A deazaflavin-dependent nitroreductase (Ddn) from Mycobacterium tuberculosis catalyzes the reduction of nitroimidazoles such as PA-824, resulting in intracellular release of lethal reactive nitrogen species. The N-terminal 30 residues of Ddn are functionally important but are flexible or access multiple conformations, preventing structural characterization of the full-length, enzymatically active enzyme. The split barrel-like fold is characterized by a central six-stranded antiparallel β barrel in a Greek key topology with four α helices: A at the N terminus (the putative helix removed for Ddn structure determination), B after an extended loop between strands β3 and β4, and C and D between strands β5 and β6. The identification of these residues and the lack of classic catalytic residues in the active site suggest that Ddn functions primarily by precisely orienting PA-824 for efficient direct hydride transfer from F420 and potentially through additional transition-state stabilization.

Well-dispersed signals for 113 of 114 nonproline residues were observed by 1H-15N-HSQC NMR spectroscopy for uniformly 15N-labeled NΔ30 Ddn protein, suggesting a well-defined three-dimensional structure. This sample also showed significant chemical shift perturbation upon addition of oxidized or reduced coenzyme F420, demonstrating tight binding of the coenzyme and suggesting that this construct adopts a physiologically relevant form. As expected (Manjunatha et al., 2006a; Taylor et al., 2010), the backbone trace shows high similarity to proteins in the split barrel-like family of flavin-binding proteins. The initial structure was then used to solve the structure of the longer NΔ30 construct by molecular replacement based on a 1.55 Å data set (Apo-1 in Table 1) and of a 1.85 Å resolution NΔ33 crystal (P3221 space group; Apo-2 in Table 1). All but the first five amino-terminal residues could be built into the electron density for both crystal forms (36–151 and 39–151, respectively). The asymmetric units (ASUs) for the Apo-1 and Apo-2 crystals both contain single molecules with similar structures (root-mean-square deviation [rmsd] is 0.96 Å). This alignment omits 14 of 113 shared Cα atoms because of conformational differences in the same regions that differ upon coenzyme binding. In Apo-1 and Apo-2, α helix D is highly disrupted, with repositioning of residues 129–144 relative to the holo-enzyme structures complementing movement of the post-β3 loop. In Apo-1, the side chain of Y136 is flipped away from the F420 binding site, with the oxygen atom moving 19 Å relative to the Holo-1 structure.

> GRNDGEGLGGTFQKIPVALLTTTGRKTGQPRVNPLYFLRDGGRVIVAASKGGAEKNPMWYLNLKANPKVQVQIKKEVLDLTARDATDEERAEYWPQLVTMYPSYQDYQSWTDRTIPIVVCEP>[2x]MVLYFIGLGLYDERDITVKGMEIAKKCDYVFAEFYTSLMAGTTLGRIQKLIGKEIRVLSREDVELNFEN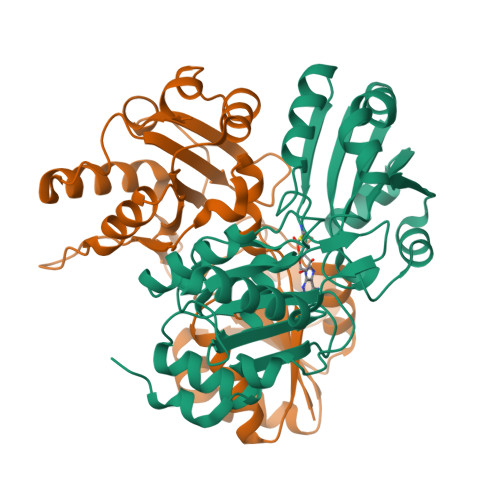IVLPLAKENDVAFLTPGDPLVATTHAELRIRAKRAGVESYVIHAPSIYSAVGITGLHIYKFGKSATVAYPEGNWFPTSYYDVIKENAERGLHTLLFLDIKAEKRMYMTANEAMELLLKVEDMKKGGVFTDDTLVVVLARAGSLNPTIRAGYVKDLIREDFGDPPHILIVPGKLHIVEAEYLVEIAGAPREILRVNV2,2,2-trifluoro-N-[(1R,2R,3R,4R,5R,6R)-2,3,5,6-tetrahydroxy-4-(hydroxymethyl)cyclohexyl]acetamide 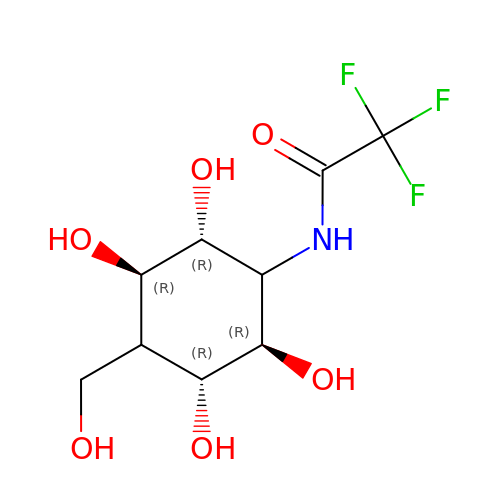| C9 H14 F3 N O6 | RPAYCNWWSJECNN-ZGGPPPIHSA-N>SMKIDVVTIFPEYLQPVRQSLPGKAIDAGLVDVAVHDLRRWTHDVHKSVDDSPYGGGPGMVMKPTVWGDALDEICTSETLLVVPTPAGYPFTQETAWQWSTEDHLVIACGRYEGIDQRVADDAATRMRVREVSIGDYVLN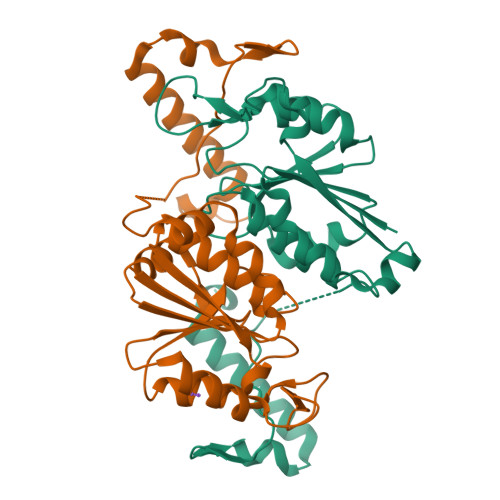GGEAAALVIIEAVLRLVPGVLGNALSAQEDSHSEGMASLLEGPSYTRPPSWRGMDVPPVLLSGDHAKIAAWRAEQSRQRTIERRPDLLGFDSP[2x]>[4x]SITENTSWNKEFSAEAVNGVFVLCKSSSKSCATNDLARASKEYLPASTFKIPNAIIGLETGVIKNEHQVFKWDGKPRAMKQWERDL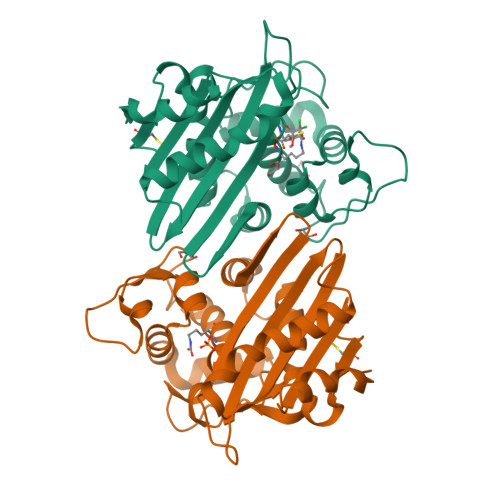TLRGAIQVSAVPVFQQIAREVGEVRMQKYLKKFSYGNQNISGGIDKFWLEGQLRISAVNQVEFLESLYLNKLSASKENQLIVKEALVTEAAPEYLVHSKTGFSGVGTESNPGVAWWVGWVEKETEVYFFAFNMDIDNESKLPLRKSIPTKIMESEGIIGG> MLEKFCNSTFWNSSFLDS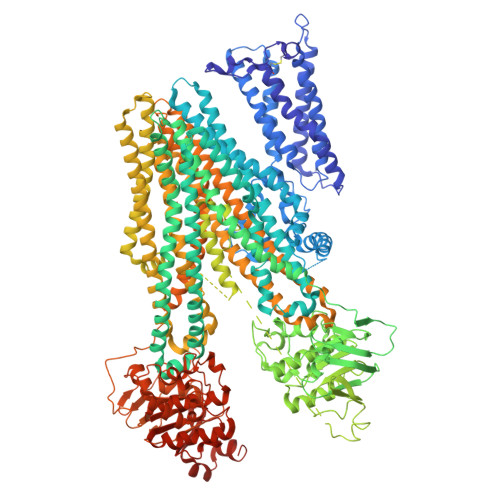PEADLPLCFEQTVLVWIPLGYLWLLAPWQLLHVYKSRTKRSSTTKLYLAKQVFVGFLLILAAIELALVLTEDSGQATVPAVRYTNPSLYLGTWLLVLLIQYSRQWCVQKNSWFLSLFWILSILCGTFQFQTLIRTLLQGDNSNLAYSCLFFISYGFQILILIFSAFSENNESSNNPSSIASFLSSITYSWYDSIILKGYKRPLTLEDVWEVDEEMKTKTLVSKFETHMKRELQKARRALQRRQEKSSQQNSGARLPGLNKNQSQSQDALVLEDVEKKKKKSGTKKDVPKSWLMKALFKTFYMVLLKSFLLKLVNDIFTFVSPQLLKLLISFASDRDTYLWIGYLCAILLFTAALIQSFCLQCYFQLCFKLGVKVRTAIMASVYKKALTLSNLARKEYTVGETVNLMSVDAQKLMDVTNFMHMLWSSVLQIVLSIFFLWRELGPSVLAGVGVMVLVIPINAILSTKSKTIQVKNMKNKDKRLKIMNEILSGIKILKYFAWEPSFRDQVQNLRKKELKNLLAFSQLQCVVIFVFQLTPVLVSVVTFSVYVLVDSNNILDAQKAFTSITLFNILRFPLSMLPMMISSMLQASVSTERLEKYLGGDDLDTSAIRHDCNFDKAMQFSEASFTWEHDSEATVRDVNLDIMAGQLVAVIGPVGSGKSSLISAMLGEMENVHGHITIKGTTAYVPQQSWIQNGTIKDNILFGTEFNEKRYQQVLEACALLPDLEMLPGGDLAEIGEKGINLSGGQKQRISLARATYQNLDIYLLDDPLSAVDAHVGKHIFNKVLGPNGLLKGKTRLLVTHSMHFLPQVDEIVVLGNGTIVEKGSYSALLAKKGEFAKNLKTFLRHTGPEEEATVHDGSEEEDDDYGLISSVEEIPEDAASITMRRENSFRRTLSRSSRSNGRHLKSLRNSLKTRNVNSLKEDEELVKGQKLIKKEFIETGKVKFSIYLEYLQAIGLFSIFFIILAFVMNSVAFIGSNLWLSAWTSDSKIFNSTDYPASQRDMRVGVYGALGLAQGIFVFIAHFWSAFGFVHASNILHKQLLNNILRAPMRFFDTTPTGRIVNRFAGDISTVDDTLPQSLRSWITCFLGIISTLVMICMATPVFTIIVIPLGIIYVSVQMFYVSTSRQLRRLDSVTRSPIYSHFSETVSGLPVIRAFEHQQRFLKHNEVRIDTNQKCVFSWITSNRWLAIRLELVGNLTVFFSALMMVIYRDTLSGDTVGFVLSNALNITQTLNWLVRMTSEIETNIVAVERITEYTKVENEAPWVTDKRPPPDWPSKGKIQFNNYQVRYRPELDLVLRGITCDIGSMEKIGVVGRTGAGKSSLTNCLFRILEAAGGQIIIDGVDIASIGLHDLREKLTIIPQDPILFSGSLRMNLDPFNNYSDEEIWKALELAHLKSFVASLQLGLSHEVTEAGGNLSIGQRQLLCLGRALLRKSKILVLDEATAAVDLETDNLIQTTIQNEFAHCTVITIAHRLHTIMDSDKVMVLDNGKIIECGSPEELLQIPGPFYFMAKEAGIENVNSTKFLEDYKDDDDKVEHHHHHHHH>[3x]MVKSLQLAHQLKDKRILLIGGGEVGLTRLYKLMPTGCKLTLVSPDLHKSIIPK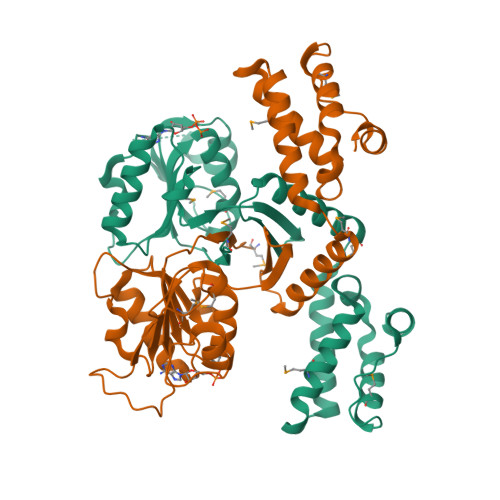FGKFIQNKDQPDYREDAKRFINPNWDPTKNEIYEYIRSDFKDEYLDLENENDAWYIIMTCIPDHPESARIYHLCKERFGKQQLVNVADKPDLCDFYFGANLEIGDRLQILISTNGLSPRFGALVRDEIRNLFTQMGDLALEDAVVKLGELRRGIRLLAPDDKDVKYRMDWARRCTDLFGIQHCHNIDVKRLLDLFKVMFQEQNCSLQFPPRERLLSEYCSS> V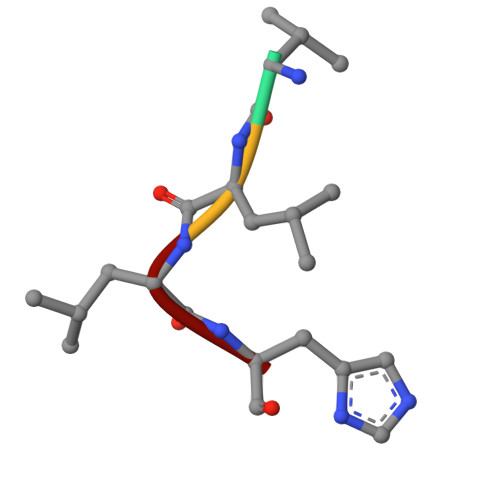LLH> MVKIYLIEHVIGAVAYDENGNIVDYITNPRDLGKITEELLNNEKGIPFSATVELLKKVNPQEVVVENEAEVPKLQALGYRVSYEPYSKVSRIFRESLPKVAIDIKFASNEEDYYNFLHELSLEYTRRKLRSAAQKRDLLAIQAVRAMDDIDKTINLFSERLREWYSIHFPELDKLIEDHEEYATIVSRFGDRGFLTIDSLKELGFNEQRINRILDAAKKSIGADISEDDLSAMRMIANTILDLYNIRRNLNNYLEGVMKEVAHHHHHH;> MA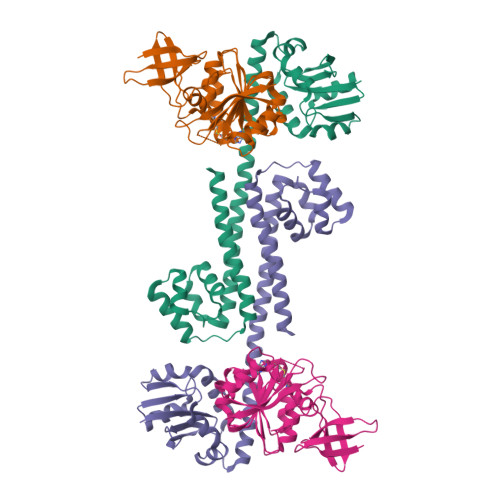EVITVKQTNMENIYECEFNDGSFRLCTRNLVPNFNVYGERLIKYEGVEYREWNAFRSKLAGAILKGLKTNPIRKGTKVLYLGAASGTTISHVSDIIELNGKAYGVEFSPRVVRELLLVAQRRPNIFPLLADARFPQSYKSVVENVDVLYVDIAQPDQTDIAIYNAKFFLKVNGDMLLVIKARSIDVTKDPKEIYKTEVEKLENSNFETIQIINLDPYDKDHAIVLSKYKG[(1~{S},2~{R},3~{S},4~{S},5~{R},6~{S})-2-(hydroxymethyl)-3,4,5,6-tetrakis(oxidanyl)cyclohexyl] 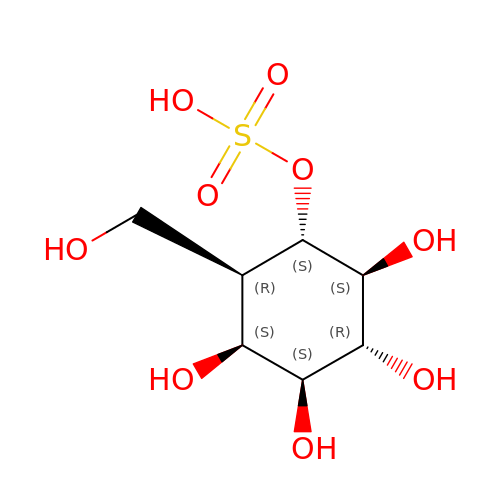hydrogen sulfate | C7 H14 O9 S | PDBNIRCVRHFXAD-ADTCQYHUSA-N>SDININLQRKSVVLGSKSNASVKFKEKLNADSITLNFMCYDMPLEATLNYNEKTDSYEGVINYNKDPEYLNVWELQSIKINGKDEQKVLNKEDLESMGLNLKDYDVTQEFIISDANSTKAVNEYMRKTSAPVKKLAGATRFETAVEISKQGWKDGSSKVVIVNGELAADGITATPLASTYDAPILLANKDDIPESTKAELKRLNPSDVIIIGDDGSVSQKAVSQIKSAVNVNVTRIGGVDRHETSLLIAKEIDKYHDVNKIYIANGYAGEYDALNISSKAGEDQQPIILANKDSVPQGTYNWLSSQGLEEAYYIGGSQSLSSKIIDQISKIAKNGTSKNRVSGADRHETNANVIKTFYPDKELSAMLVAKSDIIVDSITAGPLAAKLKAPILITPKTYVSAYHSTNLSEKTAETVYQIGDGMKDSVINSIASSLSKHNAPTEPDNSGSAAGKTVVIDPGHGGSDSGATSGLNGGAQEKKYTLNTALATTEYLRSKGINVVMTRDTDKTMALGERTALSNTIKPDLFTSIHYNASNGSGNGVEIYYKVKDKNGGTTKTAASNILKRILEK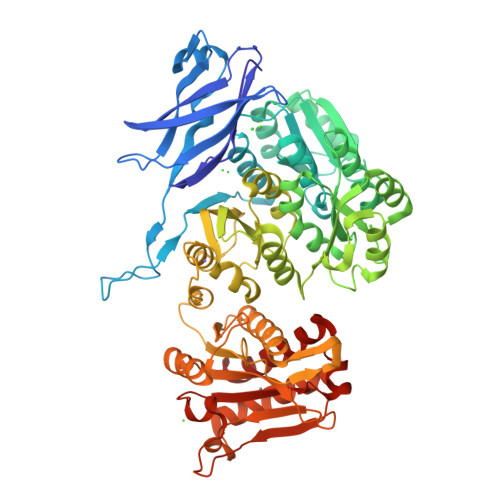FNMKNRGIKTRTLDNGKDYLYVLRNNNYPAILVECAFIDNKSDMDKLNTAEKVKTMGTQIGIGIEDTVK[2x]> TPLGPARSLPQSFLLKCLEQVRKIQADGAELQERLCAAHKLCHPEELMLLRHSLGIPQAPLSSCSSQSLQLRGCLNQLHGGLFLYQGLLQALAGISPELAPTLDTLQLDVTDFATNIWLQMEDLGAAPAVQPTQGAMPTFT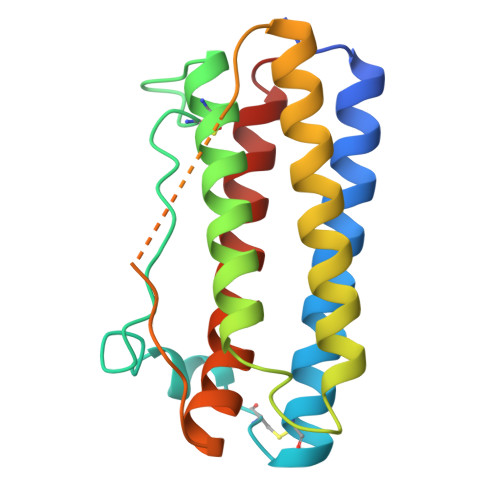SAFQRRAGGVLVASQLHRFLELAYRGLRYLAEP In S. cerevisiae meiosis I, sister kinetochores are fused through the action of the kinetochore-binding monopolin complex, and together bind a single microtubule. The conserved core of the monopolin complex comprises two nucleolar proteins, Csm1 and Lrs4. These proteins form a distinctive V-shaped complex, with two Csm1 homodimers bridged at their coiled-coil N-termini by a pair of Lrs4 subunits, thereby positioning two pairs of Csm1 globular-domain “heads” ~ 10 nm apart at the apices of the V. Each Csm1 globular domain has a conserved hydrophobic cavity implicated in binding the kinetochore protein Dsn1, leading to the proposal that monopolin could bridge Dsn1 molecules from sister kinetochores to physically fuse the kinetochores. A ~ 40-residue region within the disordered N-terminus of the core kinetochore protein, Dsn1, has been identified as the kinetochore receptor for the monopolin subunit Csm1.

Dsn1 Box 3 contains two serine residues (Sc Dsn1 S109 and S110) that are highly conserved throughout budding yeast. The high conservation and physical proximity of these serine residues to positively charged residues on Csm1 suggests that these residues may become phosphorylated, and that phosphorylation could reinforce the observed binding mode between Dsn1 Box 2-3 and Csm1. Indeed, mass spectrometry of Dsn1 purified from metaphase I-arrested cells showed that S109 and S110 are phosphorylated in vivo. Further supporting this idea, we could reconstitute a complex of Cg Csm169–181 and a minimised Cg Dsn1 Box 2-3 construct (residues 43–67) with both S66 and S67 (equivalent to Sc Dsn1 S109 and S110) mutated to aspartate to mimic phosphorylation (referred to as Cg Csm169–181:Dsn143-67DD). We determined a 1.8 Å-resolution structure of this complex, which closely agrees with both structures described above with the addition of a specific interaction between Dsn1 residue D66 and Csm1 K172. Consistent with the idea that phosphorylation of Dsn1 Box 3 promotes Csm1 binding, we found that Sc Dsn171–110 with the phosphomimetic S109D/S110D mutation showed increased binding to Sc Csm169–190 in vitro. A recent study has shown that Dsn1 Box 1 is dispensable for binding to Csm1 as measured by yeast two-hybrid assay, and our own biochemical reconstitutions reveal that the Box 2-3 region alone binds stably to Csm1, at least when the conserved Box 3 serine residues are mutated to aspartate. We hypothesise that sister kinetochore binding by the two Csm1 heads could trigger a switch in interaction mode between Box 1 and Box 2-3, with further stabilisation of the Box 2-3 interaction coming through phosphorylation of the two conserved serine residues in Box 3 (Sc Dsn1 S109 and S110).

> SNAETIEIIKDLFEHLCGVRVHRTYEDDTGLWFDTSQGSKNGIMDYKLGFVKSQAENTTEVDTEVIYVPLLKQRTAEELQELQKKLPDYLFETLSFPLRSLNQFYIKMSKSLNKKV;> SNAPTLGERLDSLHEIKSARRMDHFNDD>MSGELRVRRASSWELDLILKEAEKYGELLHEFFCVVEGKYRDVYAVNEEVWKIIEDINMRPYSLGTFVGTIRVDENLVEKFYPNLEFFSLIKLEKNYVILGPKASFLFTTGKDAPKEAVREIKWQGSKR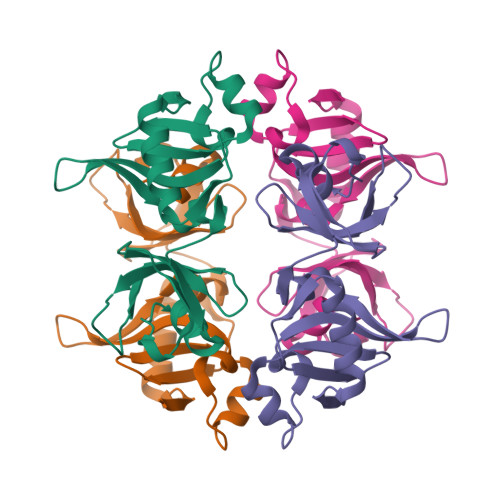VVVLNDLGDIIGIGLINPKSDRRFIKNLKDVGEFLRR[2x]> MEKLRKFFREVIAEAKKISWPSRKELLTSFGVVLVILAVT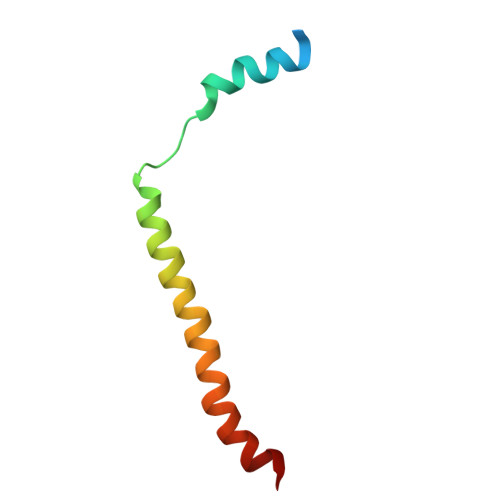SVYFFVLDFIFSGVVSAIFKALGIG>[2x]MPASLLRFLALAGTAVGLTTNHNHSPSCRVLPGDAAWPSSRDWAKLNKTLNGHLIATVPQASVCHKSPFGQYDAQACEELKSSWDISTITHVNAPGDVLSQNFQNYSCVPFTDPSQPCQLGNYPSYVVNVTGAADVQAALKFAQKHNVRIVIKNTGHDYLGKSTGKGALSLWMHNLKSTKFIKNYKAPYYKGPAAKLGAGVEGFEAYAMANSTGHRIVGGTCPTVGIVGGYTQGGGHSILSSSYGVAADNVLEWEVVTADGRHLVATPTRNSDLYWALSGGGGGTFAVVLSMTARLHRDGIVGGTLLGFNDSAVGNEVYWEAVAAFHALLPDFLDGGNSFTYSVGNNSLTAYGTMPGADRDAVDRLLRPFLDDLASRGITPVVQPRVSTNYYDHFFTYLGPAPYGNAAYFPFTNSRIIPRSLVTDPKSNAVVTDLFRNISQVPAFSPFYCDSFSVADKPHPANSLHPAWRTGMLLCAPAGSWDWDASPEEMAARDRYAAETLQPMMDAATPGGSVYLNEANHLYANWKESFYGDNYARLLRVKKKYDPDSVFYVKTGVGSEVWDVDATGRLCRA

In the present study we report the discovery and the structural characterization of two novel flavoprotein oxidases from the thermophilic fungus M. thermophila. VAO-type proteins are composed of a FAD-binding domain and substrate domain. In both MtVAO615 and MtVAO713 the cofactor FAD is covalently tethered to the protein by covalent linkages.

The crystal structure of MtVAO615 with amino acid residues 27–574 was solved in two different space groups. The structure at pH 7.5 contains one monomer while the structure at pH 5.0 contains two monomers. Rcryst/Rfree are 19.5/23.5 and 23.6/28.0 respectively. As already observed by SDS-PAGE, MtVAO615 is heavily glycosylated, showing electron density in 2Fo-Fc maps for N-glycosylation at Asn47, Asn105, Asn129, Asn211, Asn310 and Asn438. As expected, MtVAO615 harbors a bicovalently linked 6-S-cysteinyl-8α-N1-histidyl FAD while MtVAO713 has a monocovalently linked 8α-methyl-N1-histidyl FAD. The groove shaped substrate binding pocket of MtVAO615 is solvent accessible and contains, besides His157 and Cys222 which tether the FAD, Tyr159, Thr221, His237, Thr341, Tyr352, Leu399, cis-Pro401, Ala402, cis-Pro403, Ala408, Phe410, Thr413, Tyr449, Asp451, Leu475 Ala477, Ala479, Glu519. On the other hand, despite having a bicovalently bound FAD cofactor, access to the active site of MtVAO615 is rather narrow. In particular, Phe410 and Tyr449 seem to create a sort of funnel. It is worth to note that Phe410 is on a loop which runs longitudinally across the active site. While this loop is further away from the active site in the other sequence-related oxidases, in MtVAO615 it leans towards the active site contributing to narrowing the cavity.Repulsive guidance molecules (RGMs) are cell surface proteins that control processes ranging from brain development to iron metabolism. RGMs can bind to the cell guidance receptor Neogenin (NEO1) and act as coreceptors for the bone morphogenetic proteins (BMPs). Structural analysis of RGMs and their complexes with NEO1 and BMP2 revealed a common RGM architecture comprising an N-terminal domain (RGMND) essential for BMP binding and a C-terminal domain (RGMCD) sufficient for NEO1 binding. Here, we determined high-resolution structures of all three human RGMs in complex with the BMP ligand growth differentiation factor 5 (GDF5) and the ternary complex of GDF5 with RGM and NEO1.

We also determined the structures of the RGMAND–GDF5 and RGMCND–GDF5 complexes. However, while the GDF5 structure in the three complexes is largely invariant, the relative orientation of the three RGMND helix bundles towards GDF5 differs. The relative position of the α3 helix differs by ∼5 Å in RGMBND–GDF5 and RGMCND–GDF5 complexes, with its N terminus being the anchor point for a rotation of RGMND. The pivot point seems to be RGMB Leu103 (RGMA Leu97, RGMC Leu101). A relative rotation around this leucine permits the side-chain of the preceding arginine (Arg100 in RGMB) to be inserted between GDF5 fingers 1 and 2 in the RGMA– and RGMB–GDF5 complexes. In the RGMCND–GDF5 complex, however, this arginine side-chain is placed above finger 2, potentially explaining the different arrangements of the RGM α3 helix. Strikingly, the superposition of GDF5-bound RGMBND and RGMCND requires translation by 5.6 Å and rotation by 15.4°. Intriguingly, mutations in the α2–α3 linker of RGMC (Gly99Val, Gly99Arg, Leu101Pro) cause iron overload and impair interactions with the closely related BMP2 (17). GDF5 interacted similarly with RGMCND (Kd 3.9 μM) and weaker with RGMAND (Kd 16.7 μM). The juvenile hemochromatosis-causing mutation, Gly99Arg, in RGMCND and a corresponding mutation, Gly101Arg, in RGMBND attenuated the interactions with GDF5, Kd > 20 μM and > 150 μM, respectively.

> MKRQGKRPSKNLKARCSRKALHVNFKDMGWDDWIIAPLEYEAFHCEGLCEFPLRSHLEPTNHAVIQTLMNSMDPESTPPTCCVPTRLSPISILFIDSANNVVYKQYEDMVVESCGCR;> ETGQCKILRCNAEYVSSTLSLRGGGSSGALRGGGGGGRGGGVGSGGLCRALRSYALCTRRTARTCRGDLAFHSAVHGIEDLMIQHNCSRQGPTAPPPPRGPALPGAGSGLPAPGTKHHHHHH> ANPLYQKHIISINDLSRDDLNLVLATAAKLKANPQPELLKHKVIASCFFEASTRTRLSFQTSMHRLGASVVGFSDSANTSLGKKGETLADTISVISTYVDAIVMRHPQEGAARLATEFSGNVPVLNAGDGSNQHPTQTLLDLFTIQQTEGRLDNLHVAMVGDLKYGRTVHSLTQALAKFDGNRFYFIAPDALAMPEYILDMLDEKGIAWSLHSSIEEVMAEVDILYMTRVQKERLDPSEYANVKAQFVLRASDLHNAKANMKVLHPLPRVDEIATDVDKTPHAWYFQQAGNG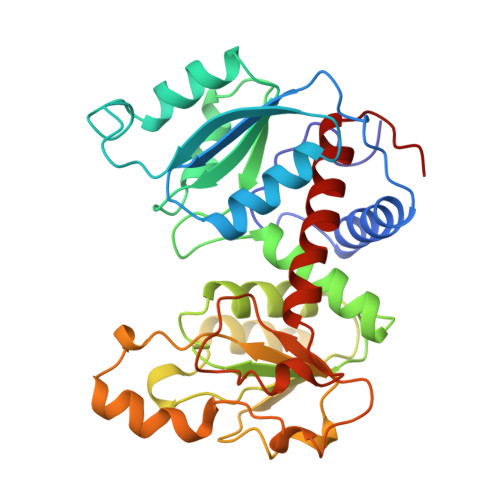IFARQALLALVLNRDLVL> MSSIQILSTTTIHAPNHPNDYSIDLTPWDLQYLTFGINQKGVLYHHPPNLDTTNQIQHLKQSLLSTLEYFHPLTGRLNVTNHEDNTVSYSVNCNNEGALFIHAEAKDISVGEILESTYLPVILYSFFPLNGVKNYQGTTKPLFAVQVTELIDGIFIGCAINHSVVDGTAFWYFINTWAKISKGDFEISPVPSFKRWFPDSVQPPIRFQFPKESQNDEEEKLCKPMFERLFHFSKENIAKLKSKANLEAGKTRISSLQAVFTHIWRAIVRSRSVDPQEELKFGIDIGVRPRLTPPRKNDYFANAVVECAVTMKAGELLEDGGLGKGAWEMNQK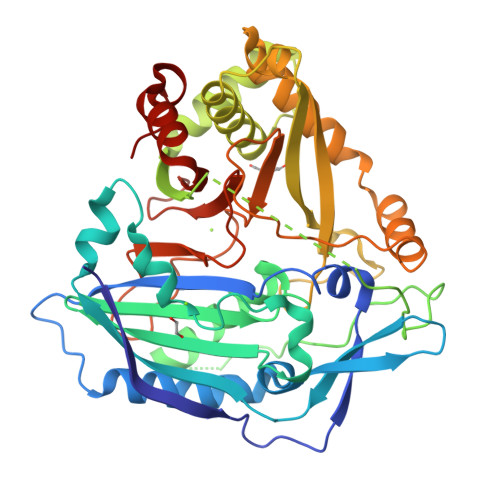IALYNDEMVKNLFENWSTTPSFSFLGSNLADSNSVMIGSSPWFDVYGNDFGWGKPVGVRNGGTNKRNWKVYVCAGVEEGSMNLEVCLPYENLEAIGNDSEFMDAASG>TETTSFLITKFSPDQQNLIFQGDGYTTKEKLTLTKAVKNTVGRALYSSPIHIWDRETGNVANFVTSFTFVINAPNSYNVADGFTFFIAPVDTKPQTGGGYLGVFNSAEYDKTTQTVAVEFDTFYNAAWDPSNRDRHIGIDVNSIKSVNTKSWKLQNGEEANVVIAFNAATNVLTVSLTYPNNSLEEEVTSYTL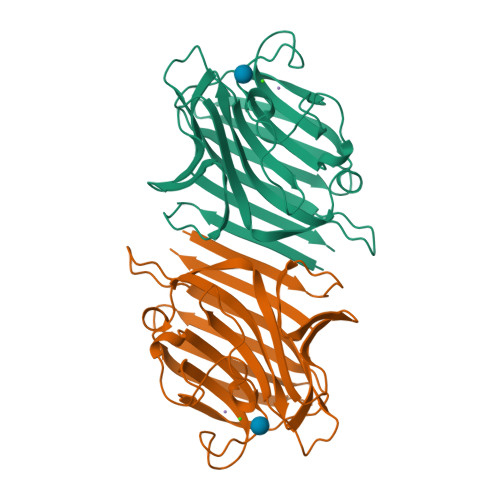SDVVSLKDVVPEWVRIGFSATTGAEYAAHEVLSWSFHSELS[2x]>[2x]SLRECELYVQKHNIQALLKDSIVQLCTARPER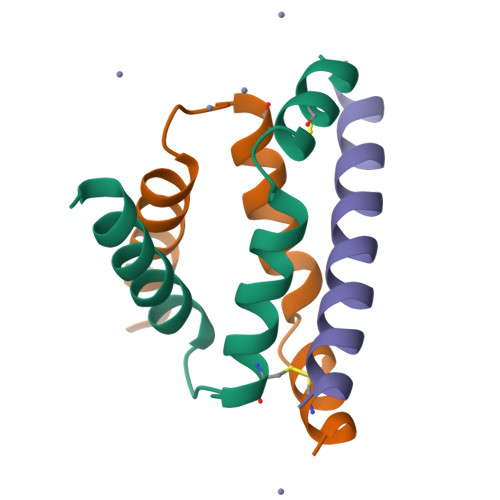PMAFLREYFEKLEKEEAK;> GSPEFVQGNTDEAQEELAWKIAKMIVSDVMQQAQYDQPLEKSTKL H5 and H12 in the 6-helix bundle are discontinuous. dimer indicates clusters of charged residues on both sides of the membrane. transported by PaNhaP, K+ is not. structure thus serves as an excellent model for the membrane part of NHE1.

but unlike K+, Tl+ is a substrate of PaNhaP. Tl+ is able to replace Na+ in PaNhaP. the main-chain carbonyl of Thr129 coordinate the substrate ion. Glu154 and Asn158 is not directly involved in ion coordination. ion via a bound water molecule. molecule next to Tl+ is green. surface and ∼22 Å from the extracellular surface. structure shows the inward-open conformation of PaNhaP. Tl+ may account for the lower transport rate in PaNhaP.

>MIELSLAEALFLILFTGVISMLISRRTGISYVPIFILTGLVIGPLLKLIPRDLAHEIFDFVRVFGLVIILFTEGHNLSWRLLKKNMPTIVTLDTIGLILTALIAGFIFKVVFNSSFLLGFLFGAIIGATDPATLIPLFRQYRVKQDIETVIVTESIFNDPLGIVLTLIAISMLVPGYGGGIFSTLSEKLGIYAGGVIYFLYNVSVSISLGIFLGILGYKFIKRTGIFDFPEIEAFSLSLAFLGFFIGERLDASGYLVATVTGIVLGNYKLLKPRENIRILKRLQRAIEKEVHFNDTLAALATIFIFVLLGAEMNLEVIWSNLGKGLLVALGVMILARPLATLPLLKWWNFREYLFIALEGPRGVVPSALASLPLSLALKYKSPLLTVHWGEIIMATVVITVLTSVIVETLWIPILKDKLD[2x]>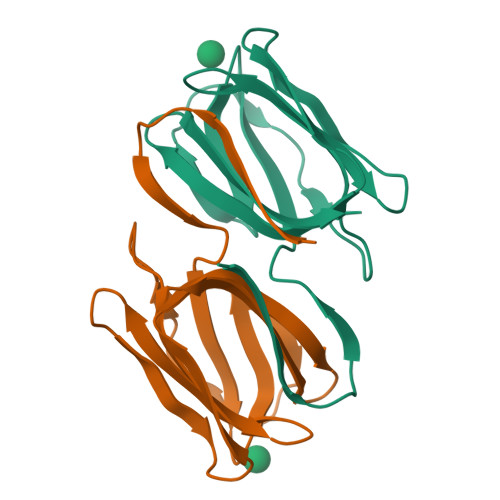[2x]MGGSSHHHHHHSSGLVPRGSGGLTHRKFGGSGGSPFSGLSSIAVRSGSWLDAIIIDGVHHGGSGGNLSPTFTFGSGEYISNMTIRSGDYIDNISFETNMGRRFGPYGGSGGSANTLSNVKVIQINGSAGDYLDSLDIYYEQY> ALTAKHRPSVVWLHNAECT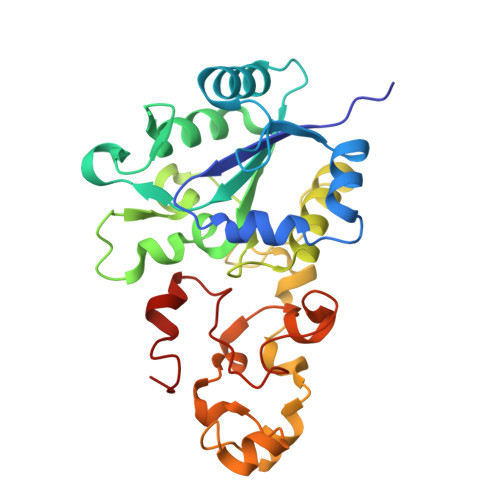GCTEAAIRTIKPYIDALILDTISLDYQETIMAAAGEAAEAALHQALEGKDGYYLVVEGGLPTIDGGQWGMVAGHPMIETTKKAAAKAKGIICIGTCSAYGGVQKAKPNPSQAKGVSEALGVKTINIPGCPPNPINFVGAVVHVLTKGIPDLDENGRPKLFYGELVHDNCPRLPHFEASEFAPSFDSEEAKKGFCLYELGCKGPVTYNNCPKVLFNQVNWPVQAGHPCLGCSEPDFWDTMTPFYEQG> MAAASTEGVISNKQVILKDYVTGFPKESDMQLTTATTKLKLPEGSK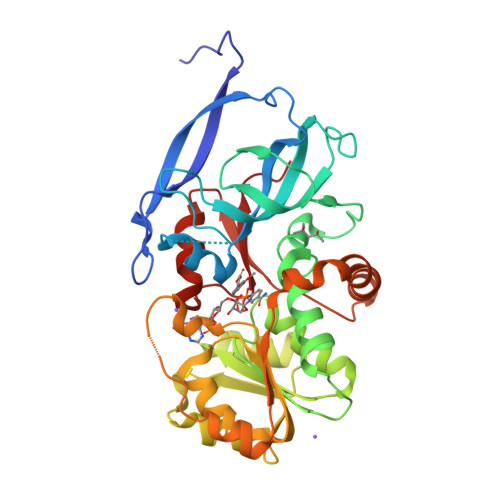GVLVKNLYLSCDPYMRSRMTKREPGASYAASFDAGSPIVGYGVAKVLESGDPKFKKGDLIWGMTGWEEYSVITSTESLFKIQHIDVPLSYYTGILGMPGMTAYAGFYEICNPKKGETVFVSAASGAVGQLVGQFAKLLGCYVVGSAGSKEKVDLLKNKFGFDNAFNYKEEPDLDAALKRYFPEGIDIYFENVGGVMLDAVLPNMRVHGRIAVCGLISQYNIDEPEGCHNLMYLIIKQVRMQGFLVFSYYHLYEKFLEMVLPAIKEGKLTYVEDVVEGLESAPAALIGLYAGRNVGKQVVVVSRE>[2x]CQDPTIFEERHLKYISQLGKGNFGSVELCRYDPLGDNTGALVAVKQLQHSGPDQQRDF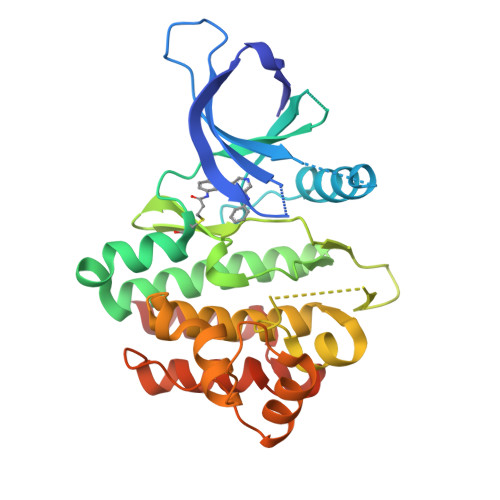QREIQILKALHSDFIVKYRGVSYGPGRQSLRLVMEYLPSGCLRDFLQRHRARLDASRLLLYSSQICKGMEYLGSRRCVHRALAARNILVESEAHVKIADFGLAKLLPLDKDYYVVREPGQSPIFWYAPESLSDNIFSRQSDVWSFGVVLYELFTYCDKSCSPSAEFLRMMGSERDVPALSRLLELLEEGQRLPAPPACPAEVHELMKLCWAPSPQDRPSFSALGPQLDMLWSGSR>[4x]MDLTINYKSTLGDDVAAYIYKETNK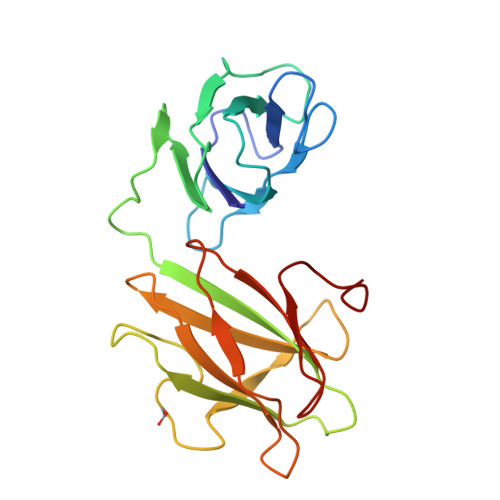PAGEWPGKTMTATAGHEGWYTMHLTLDNSTDYSLILNDDGHGNQLKDVTLSTKGKAEAEYWFDGSLSETKPADWKYVTTIHYLASGMGSTIYNYMWGADASATGAGVGKEWPGGQISANADHLGWYDVVYTQDVKQNFSCIFNNNNGTQTDNIDVSVTSTSTELWVTGTKGDTTVYKTAPDSWE>[2x]MMENIMKKRLLSTSISTL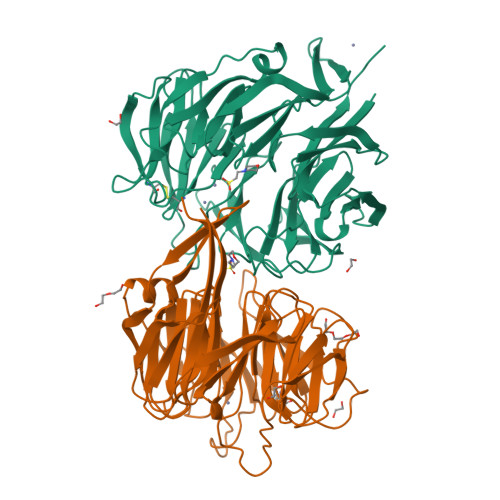LLGLSVMPAFADEDVTAWRLFIADHDKPVVNVIDALDGDKLATFNVKGPANLSRSESGATIFAIQGSAGVVSTIASGIAFHDHGDHADIDIDAPKLLPLELTGKKPGHFVERQGKIAQWFDGEDSAQILGESAVLKGQKNITKVNVVAPHHGVAVPYDNYAVVSIPNPDDASKRPVGARVVDLQGKKVGDDALCPGLHGSAGSGDTFALSCETGLLLITQKNAAPVIRHLPYAKTLPEGSTSTLIGGKGMQYFIGNYGPDRIILVDPTESDSFRLIQLPTRRVHFVVDPVRAKFAYVFTEDGKLNQIDVLKGEISQSVRVTDPYSMDGHWNDPRPRIAVADNKIYVTDPLKSKIIVLDATSFKKTSEISVEGQPFNIVAVGGSGKVHGEHHDHEAHHHDDHAH>GVHSFWDIAGPTARPVRLESLEDKRMAVDASIWIYQFLKAVRDQEGNAVKNSHITGFFRRICKLLYFGIRPVFVFDGGVPVLKRETIRQRKERRQGKRESAKSTARKLLANTTLSTSAERNVAENAFVEDELFEQQMKDKRDSDEVTMDMIKEVQELLSRFGIPYITAPMEAEAQCAELLQLNLVDGIITDDSDVFLFGGTKIYKNMFHEKNYVEFYDAESILKLLGLDRKNMIELAQLLGSDYTNGLKGMGPVSSIEVIAEFGNLK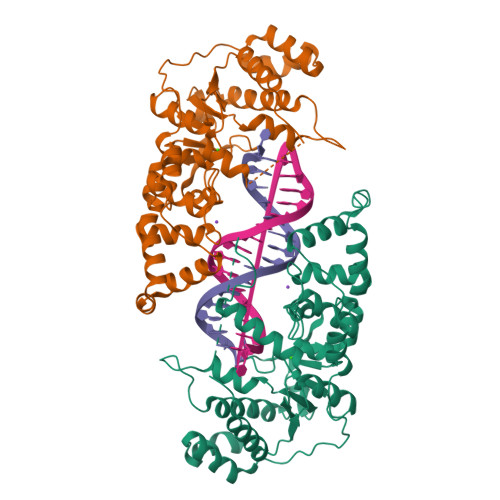NFKDWYNNGQFDKRKQETENKFEKDLRKKLVNNEIILDDDFPSVMVYDAYMRPEVDHDTTPFVWGVPDLDMLRSFMKTQLGWPHEKSDEILIPLIRDV[4x]>MASMTGGQQMGAPITAYAQQTRGLLGCIITSLTGRDKNQVEGEVQIVSTATQTFLATCINGVCWTVYHGAGTRTIASPKGPVIQMYTNVDQDLVGWPAPQGSRSLTPCTCGSSDLYLVTRHADVIPVRRRGDSRGSLLSPRPISYLKGSSGGPLLCPAGHAVGLF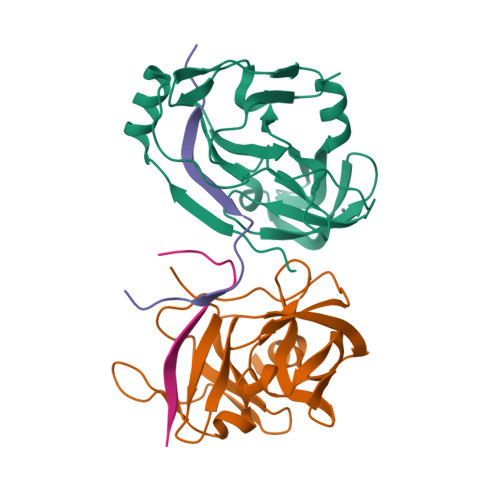RAAVCTRGVAKAVDFIPVENLETTMRSGSHHHHHH[2x];>[2x]KKGCVVIVGRIVLSGKPAIIPKK>MTIKNFTFFSPNSTEFPVGSNNDGKLYMMLTGMDYRTIRRKD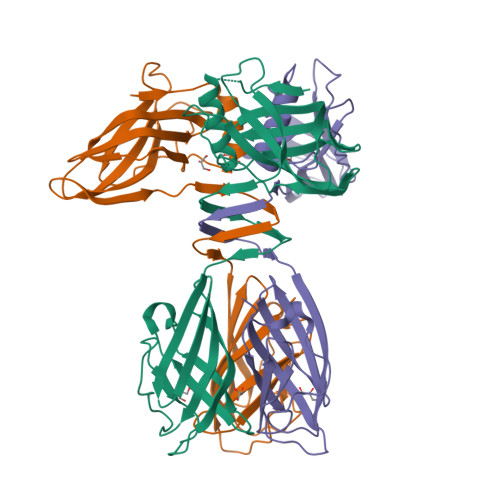WSSPLNTALNVQYTNTSIIAGGRYFELLNETVALKGDSVNYIHANIDLTQTANPVSLSAETANNSNGVDINNGSGVLKVCFDIVTTSGTGVTSTKPIVQTSTLDSISVNDMTVSGSIDVPVQTLTVEAGNGLQLQLTKKNNDLVIVRFFGSVSNIQKGWNMSGTWVDRPFRPAAVQSLVGHFAGRDTSFHIDINPNGSITWWGANIDKTPIATRGNGSYFIK[3x]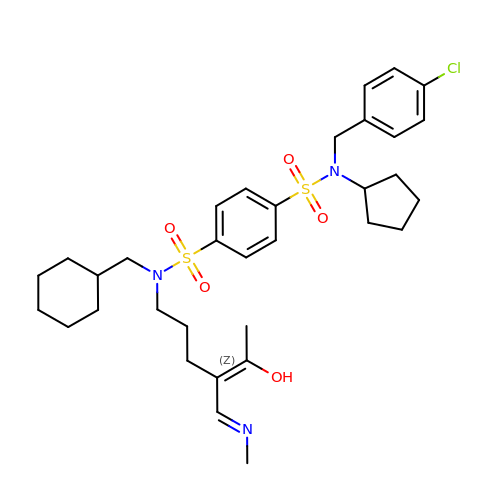~{N}4-[(4-chlorophenyl)methyl]-~{N}1-(cyclohexylmethyl)-~{N}4-cyclopentyl-~{N}1-[(~{Z})-4-[(~{E})-methyliminomethyl]-5-oxidanyl-hex-4-enyl]benzene-1,4-disulfonamide | C33 H46 Cl N3 O5 S2 | BJGXSIOLQNSMNV-ATLOAHSKSA-N>[2x]GSHMASMRVVKELEDLQKKPPPYLRNLSSDDANVLVWHALLLPDQPPYHLKAFNLR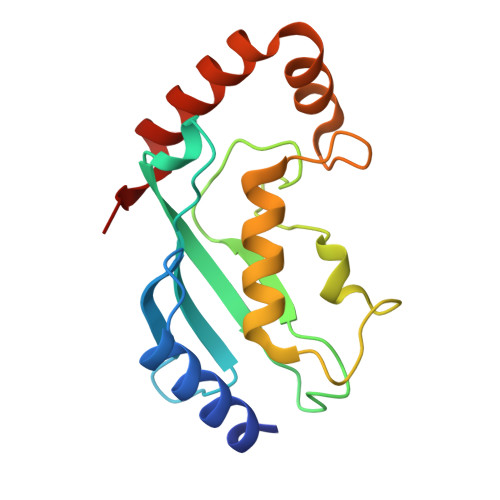ISFPPEYPFKPPMIKFTTKIYHPNVDENGQICLPIISSENWKPCTKTCQVLEALNVLVNRPNIREPLRMDLADLLTQNPELFRKNAEEFTLRFGVDRPS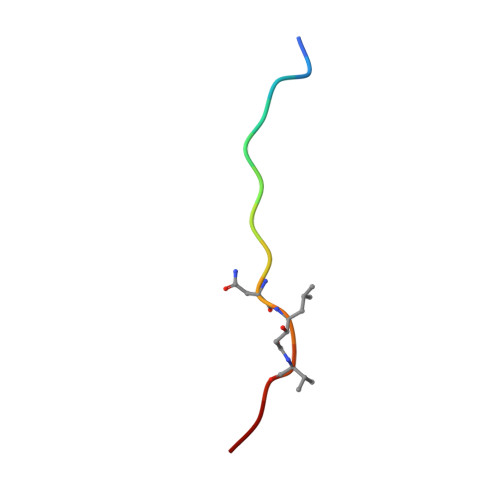> KTEEISEVNXVAEF>MAEAASCARKGTKYAEGTQPFTVLIEGNIGSGKTTYLNHFEKYKNDICLLTEPVEKWRNVNGVNLLELMYKDPKKWAMPFQSYVTLTMLQSHTAPTNKKLKIMERSIFSARYCFVENMRRNGSLEQGMYNTLEEWYKFIEESIHVQADLIIYLRT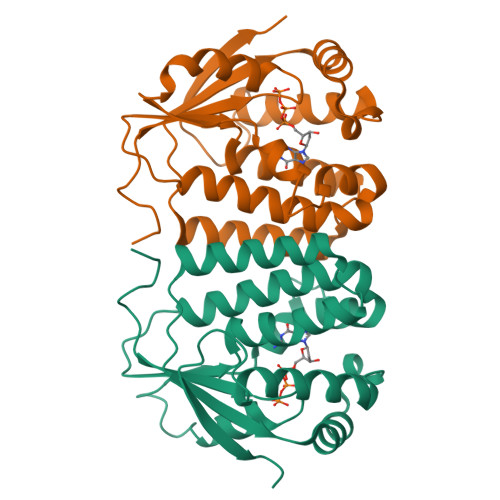SPEVAYERIRQRARSEESCVPLKYLQELHELHEDWLIHQRRPQSCKVLVLDADLNLENIGTEYQRSESSIFDAIS[2x]> NMSSGGRGGIDISTELS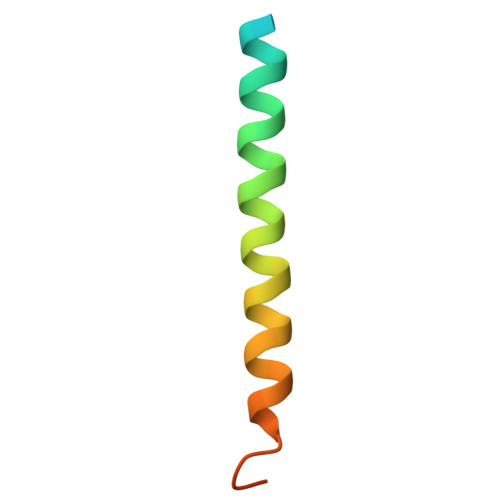KVNASLQNTVKYIKESNHQLQSVIVNSKIGA> AQSVPWGISRVQAPAAHNRGLTGSGVKVAVLDTGISTHPDLNIRGGASFVPGEPSTQDGNGHGTHVAGTIAALNNSIGVLGVAPSAELYAVKVLGASGSGSVSSIAQGLEWAGNNGMHV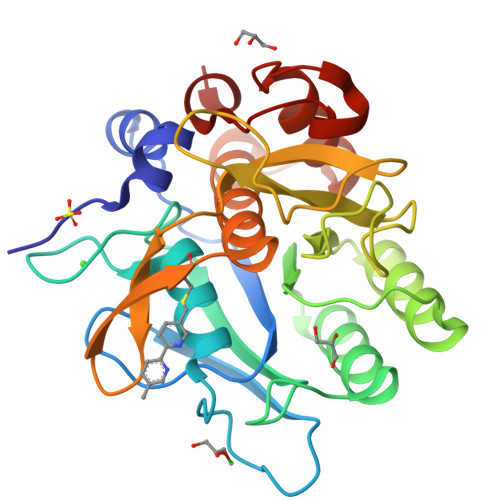ANLSLGSPSPSATLEQAVNSATSRGVLVVAASGNSGAGSISYPARYANAMAVGATDQNNNRASFSQYGAGLDIVAPGVNVQSTYPGSTYASCNGTSMATPHVAGAAALVKQKNPSWSNVQIRNHLKNTATSLGSTNLYGSGLVNAEAATR> MNEASSKFVDNIAIEKLLNEKLLRVSHRPKNLFYDDEKVFDDLCKCETDMSKVKLAEGDKNLKRFEFPSFLKTEEYIENNIVYLYYHPAKDPVCNILLLHGLYDDNMLNYGFLTRMLNELKFNVFLMELPFHFNRKPAESFFSGEYFISADLLRARNAFIQSIYDIEASRNLIGNINTLPCLLVGFSMGGCISFRYHMLRDSFKGTFLINPVTDMLLLVWDNPLLVKVKKDLEDSGVGKEQVMDVFRIIDPCENINTRFNTDNIA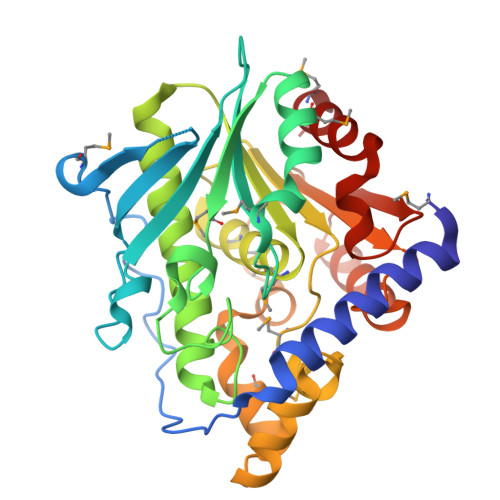VVYSIYDQIVGEEKNAIFVEKIKKAGLKKILEYHAGHLNILRVPKLSNDIYEFFMSCL Synaptic vesicle glycoprotein 2a (SV2A), a putative membrane transporter in the synaptic vesicles (SVs), has been identified as a target of LEV and BRV. SV2A also serves as a receptor for botulinum neurotoxin (BoNT), which is the most toxic protein and has paradoxically emerged as a potent reagent for therapeutic and cosmetic applications. SV2 family proteins belong to the major facilitator superfamily (MFS) with 12 predicted transmembrane helices. In addition to the transmembrane domain (TMD) core, a cytosolic N-terminal region and a large fourth luminal domain (LD4) are present.

Purified HCA2 was mixed with purified SV2A to form a complex, and then LEV was added. We used cryo-EM single-particle reconstruction to determine the structure of the SV2A–HCA2–LEV complex. We successfully reconstructed a cryo-EM map of the SV2A–HCA2–LEV complex with a nominal resolution of 2.88 Å. The quality of the cryo-EM map is sufficient for modeling the SV2A and HCA2, except that the peripheral region of the HCA2 shows poor density. An unambiguous density, assigned as LEV, was observed at the base of the central cavity. Substrate-binding sites are typically located at the base of the central cavity of MFS transporters. Therefore, LEV is likely to occupy the binding pocket of an unidentified SV2A substrate. A narrow pathway is formed from bound LEV to the extracellular space, indicating that SV2A adopts an outward-open conformation (intravesicular-facing conformation). The γ-lactam ring of LEV creates a π–π stacking interaction with Trp300 on TM5 and Trp666 on TM10. The carboxyl and amide groups of the butanamide moiety in LEV form hydrogen bonds with the Asp670 side chain.

> MDYKDDDDKEEGFRDRAAFIRGAKDIAKEVKKHAAKKVVKGLDRVQDEYSRRSYSRFEEEDDDDDFPAPSDGYYRGEGTQDEEEGGASSDATEGHDEDDEIYEGEYQGIPRAESGGKGERMADGAPLAGVRGGLSDGEGPPGGRGEAQRRKEREELAQQYEAILRECGHGRFQWTLYFVLGLALMADGVEVFVVGFVLPSAEKDMCLSDSNKGMLGLIVYLGMMVGAFLWGGLADRLGRRQCLLISLSVNSVFAFFSSFVQGYGTFLFCRLLSGVGIGGSIPIVFSYFSEFLAQEKRGEHLSWLCMFWMIGGVYAAAMAWAIIPHYGWSFQMGSAYQFHSWRVFVLVCAFPSVFAIGALTTQPESPRFFLENGKHDEAWMVLKQVHDTNMRAKGHPERVFSVTHIKTIHQEDELIEIQSDTGTWYQRWGVRALSLGGQVWGNFLSCFGPEYRRITLMMMGVWFTMSFSYYGLTVWFPDMIRHLQAVDYASRTKVFPGERVEHVTFNFTLENQIHRGGQYFNDKFIGLRLKSVSFEDSLFEECYFEDVTSSNTFFRNCTFINTVFYNTDLFEYKFVNSRLINSTFLHNKEGCPLDVTGTGEGAYMVYFVSFLGTLAVLPGNIVSALLMDKIGRLRMLAGSSVMSCVSCFFLSFGNSESAMIALLCLFGGVSIASWNALDVLTVELYPSDKRTTAFGFLNALCKLAAVLGISIFTSFVGITKAAPILFASAALALGSSLALKLPETRGQVLQ;> KNIVNTSILSIVYKKDDLIDLSRYGAKINIGDRVYYDSIDKNQIKLINLESSTIEVILKNAIVYNSMYENFSTSFWIKIPKYFSKINLNNEYTIINCIENNSGWKVSLNYGEIIWTLQDNKQNIQRVVFKYSQMVNISDYINRWIFVTITNNRLTKSKIYINGRLIDQKPISNLGNIHASNKIMFKLDGCRDPRRYIMIKYFNLFDKELNEKEIKDLYDSQSNSGILKDFWGNYLQYDKPYYMLNLFDPNKYVDVNNIGIRGYMYLKGPRGSVVTTNIYLNSTLYEGTKFIIKKYASGNEDNIVRNNDRVYINVVVKNKEYRLATNASQAGVEKILSALEIPDVGNLSQVVVMKSKDDQGIRNKCKMNLQDNNGNDIGFIGFHLYDNIAKLVASNWYNRQVGKASRTFGCSWEFIPVDDGWGESSL>FKIETTPESRYLAQIGDSVSLTCSTTGCESPFFSWRTQIDSPLNGKVTNEGTTSTLTMNPVSFGNEHSYLCTATCESRKLEKGIQVEIYSFPKDPEIHLSGPLEAGKPITVKCSVADVYPFDRLEIDLLKGDHLMKS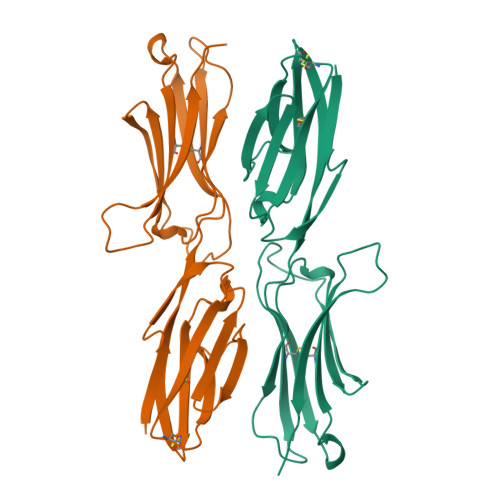QEFLEDADRKSLETKSLEVTFTPVIEDIGKVLVCRAKLHIDEMDSVPTVRQAVKELQVD[2x]>MATNAKPVYKRILLKLSGEALQGTEGFGIDASILDRMAQEIKELVELGIQVGVVIGGGNLFRGAGLAKAGMNRVVGDHMGMLATVMNGLAMRDALHRAYVNARLMSAIPLNAVCDSYSWAEAISLLRNNRVVILSAGTGNPFFTTDSAACLRGIEIEANVVLKATKVDGVFTADPAKDPTATMYEQLTYSEVL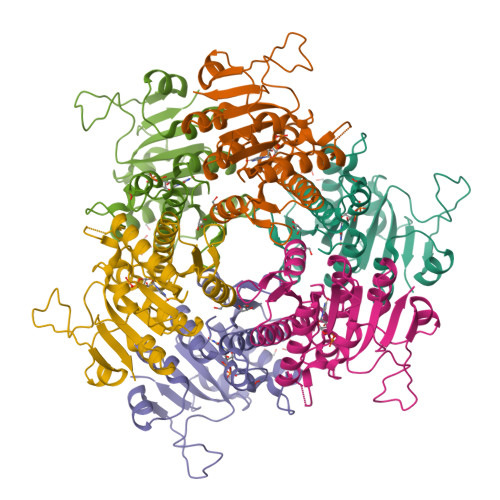EKELKVMDLAAFTLARDHKLPIRVFNMNKPGALRRVVMGEKEGTLITE[2x]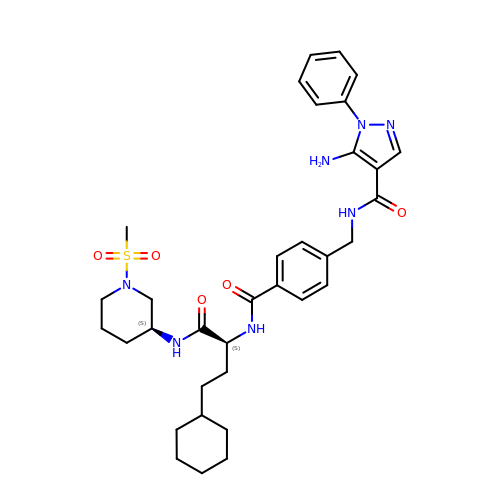5-amino-N-(4-(((2S)-4-cyclohexyl-1-((1-(methylsulfonyl)piperidin-3-yl)amino)-1-oxobutan-2-yl)carbamoyl)benzyl)-1-phenyl-1H-pyrazole-4-carboxamide | C34 H45 N7 O5 S | GODYJVJUBKYVOU-FIBWVYCGSA-N> GSPEFIAKEIMSSEKVFVDVLKLLHIDFRDAVAHASRQLGKPVIEDRILNQILYYLPQLYELNRDLLKELEERMLHW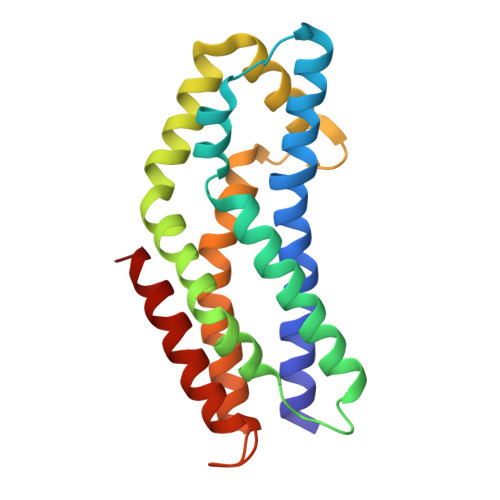TEQQRIADIFVKKGPYLKMYSTYIKEFDKNIALLDEQCKKNPGFAAVVREFEMSPRCANLALKHYLLKPVQRIPQYRLLLTDYLKNLIEDAGDYRDTQDALAVVIEVANHAN> MAPTWFYNTTNSEKLRELQHVLGGSAKLGYLTAKVTEILDVDLETVI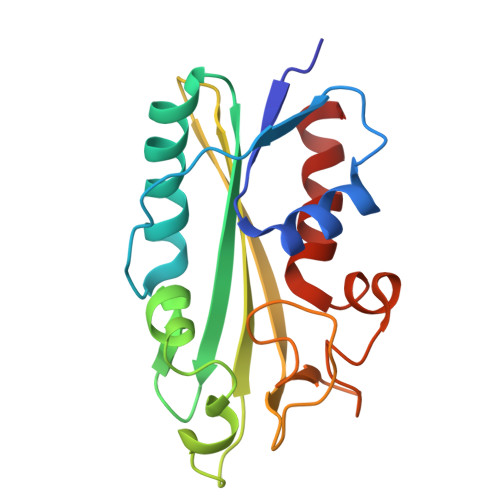RAKAIAAYRAVRVPVIVEHGALCIDALNGLPGALVKPFWESLDTRLCEVIPAGQRTARARGALCYCDGRERHVLIEETEGEIAPSARGTGGFHWDPIFIPKGQTRTFAEMSLDEKLSFSPLGRLHTRLRTELGL>XGEVAQAVKEVAKAVKEVAWAVKEVAQAVKGX[12x]

CCs are quaternary structures comprising two or more α-helices supercoiled around each other with cyclic (Cn) or dihedral (Dn) symmetry. Here, we describe variants with all combinations of the aliphatic residues, Ile, Leu and Val, at a and d to give four classes of peptide: the ββ class, with a and d = Ile or Val; Lβ, a = Leu and d = Ile or Val; βL, a = Ile or Val and d = Leu; and LL, a = d = Leu. Peptides are named systematically appending the one-letter code for the amino acids at the a and d sites to “CC-Type2-“; e.g., CC-Hept becomes CC-Type2-LI. In summary, solution-phase data and X-ray crystal structures demonstrate conclusively that different classes of Type-2 coiled-coil (CC) peptides—i.e., based on abcdefg repeats with predominantly hydrophobic residues at a, d, e and g—adopt a range of distinct states.

As a = d = β-branched specify blunt-ended α-helical barrels, we explored all four combinations of Ile and Val at these sites. CC-Type2-VV, -IV, -VI and -II, were helical and bound DPH in solution consistent with α-helical barrels. Interestingly, X-ray crystallography revealed that oligomer state increased through this series: CC-Type2-VV was hexameric; CC-Type2-IV, heptameric; and CC-Type2-II, octameric. Concomitantly, the dimensions of the internal pore diameters increased: VV, 4.8–7.7 Å; IV, 6.2–9.2 Å; and II, 9.0–11.0 Å. Finally, the modelling offers a clear explanation for why the ββ and Lβ classes exclusively form non-collapsed Cn-symmetric α-helical barrels. Sequences from both classes scored worse when threaded onto most of the slipped and collapsed structures (upper-right-hand regions of Fig. 7e). More specifically, by disfavouring alternative states, potential steric clashes involving β-branched Ile residues at a and d appear critical for maintaining parallel α-helical-barrels structures.>[8x]MPVDKNLRDLEPGIHTDLEGRLTYGGYLRLDQLLSAQQPLSEPAHHDEMLFIIQAQTSELWLKLLAHELRAAIVHLQRDEVWQCRKVLARSKQVLRQLTEQWSVLETLTPSEYMGFRDVLGPSSGFQSLQYRYIEFLLGNKNPQMLQV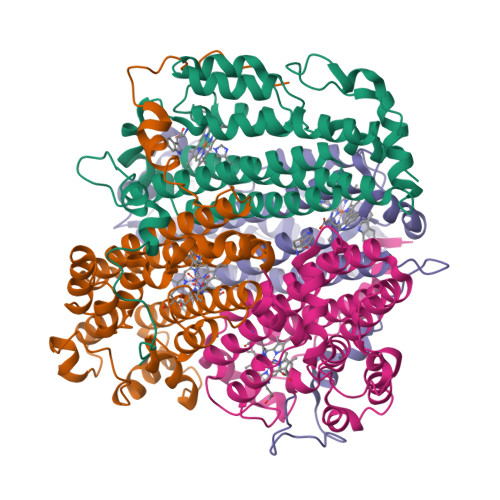FAYDPAGQARLREVLEAPSLYEEFLRYLARFGHAIPQQYQARDWTAAHVADDTLRPVFERIYENTDRYWREYSLCEDLVDVETQFQLWRFRHMRTVMRVIGFKRGTGGSSGVGFLQQALALTFFPELFDVRTSVGVDNRPPQGSADAGKRLEHHHHHH>[2x]MFTGIVQGTAKLVSIDEKPNFRTHVVELPDHMLDGLETGASV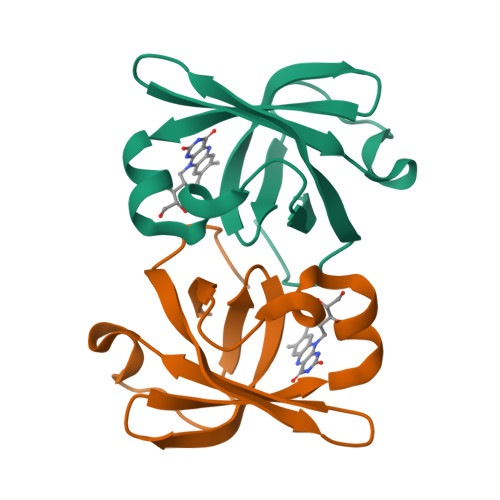AHNGCCLTVTEINGNHVSFDLMKETLRITNLGDLKVGDWVNVERAAKFSDEIGGH>[4x]GSQSSERVVIGSKPFNEQYILANMIAILLEENGYKAEVKEGLGGTLVNYEALKRNDIQLYVEYTGTAYNVILRKQPPELWDQQYIFDEVKKGLLEADGVVVAAKLGFRDDYALAVRADWAEENGVEKISDLAEFADQLVFGSDPEFASRPDGLPQIKKVYGFEFKEVKQMEPTLMYEA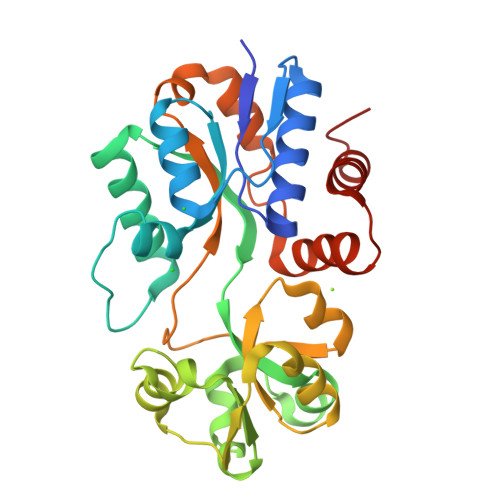IKNKQVDVIPAYTTDSRVDLFNLKILEDDKGALPPYDAIIIVNGNTAKDEKLISVLKLLEDRIDTDTMRALNYQYDVEKKDAREIAMSFLKEQGLVK1-[(4-chloranyl-2-methyl-phenyl)methyl]-3-(7,10-dioxa-13,17,18,21-tetrazatetracyclo[12.5.2.1^{2,6}.0^{17,20}]docosa-1(20),2(22),3,5,14(21),15,18-heptaen-5-yl)urea 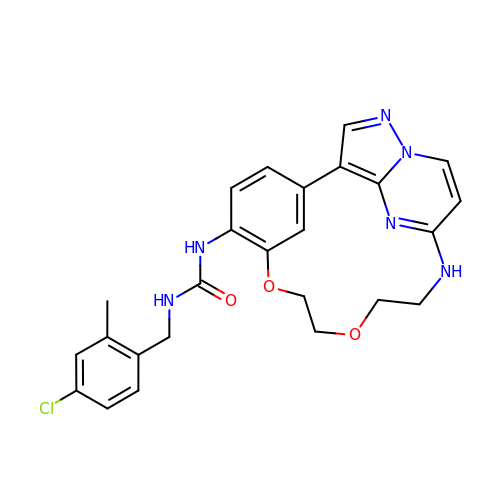| C25 H25 Cl N6 O3 | SMEVONJPJBGLLE-UHFFFAOYSA-N NbUGT72AY1 is a promiscuous transferase that glycosylates bioactive hydroxycoumarins such as scopoletin and umbelliferone, as well as monolignols involved in lignin formation and various other small molecules. Five distinct GT protein folds have been identified that are capable of GT activity (termed GT-A to GT-E). NbUGT72AY1 adopts a GT-B fold comprised of two distinct N-terminal and C-terminal Rossmann-like domains (shown in cyan and brown in Fig. 2, respectively) of seven and six parallel β-sheets, respectively linked to α-helices, connected by a linker region and an interdomain cleft. The catalytic mechanism of inverting UGT such as NbUGT72AY1 is a direct displacement bimolecular nucleophilic substitution (SN2)-like reaction enabled by an enzymatic base catalyst.

Moreover, NbUGT72AY1 crystallized in the presence of scopoletin (III), UDP (IV), and a mixture of scopoletin and the non-transferable donor UDP2FG (V). In all structures that have scopoletin bound (III, V, VI, VIII, and IX), H2 has 2-3 turns while conformers associated with UDP (IV) and UDP2FG (VII) have 4 turns. The arrangement of the Trp350 side chain in the 3D structure obtained in the presence of scopoletin (III) is clearly different. Binding of scopoletin (III) or UDP2FG (VII) results in the conversion of the loop (loop 2) between Ile42-Leu59 (green) into a helix (helix 2), but differ in the orientation of Try350 (blue) (Trp-, π interaction with uracil is not possible; Trp + , π interaction), whereas the closing loop remains flexible in both structures (yellow/red). The complexes with UDP2FG (VII_E and VII_B) show significantly more interactions within the protein than the structures with scopoletin (III), which is due to the increased number of van der Waals interactions. Starting with the apo-enzyme (I), two different conformational changes can occur after substrate binding depending on whether the acceptor (I → III) or donor (I → VII) is the first to interact with the protein. Structures III and VII differ both in the length of helix H2 and in the spatial orientation of Trp350, leading to the formation of an unproductive SI complex V and a catalytically active complex VI, respectively, after binding of the respective second substrate. High scopoletin concentrations lead to increased use of the non-productive cycle, eventually resulting in SI.

> SSQLHVAIVSSPGMGHLIPVLVLGNRLATHHNIKITILAITTTSSSAETEFLKKTTLTNEEKTIEIIPVPSVDISHLINSSTKIFTQLRLLVREALPKIHSTIASMTHRPDALIVDIFCTQILPIAEEFNISKYTYHPTTAWTLALAIYCQVFDKEIEGEYVELKEPLKIPGCKALRPDDVVDPLLDRSDQQYEEYVKLGKEYTDFDGILINTWEDLEPETINALRYNEKLRLLLKVPVFPIGPLRRKVETTLNDEVIQWLDKQNNESVLFVSFGSGGTLSTKQMTELAWGLELSQQKFVWVVRPPSDGDADSAYLNSAGKDTRDMSEYLPEGFLTRTKDMGLVVPMWANQVEILSHSSVGGFLTHCGWNSTVESLTNGVPMIAWPLHAEQKMNAAMLTEELGVAIRPAVLPTKKLVKREEIQGMVRILMQTKEGKRIKEKAKKLKKSAENALSDGGSSYNSICELVKDIRSREL> GSHMEILWNEAKAFIAECYQELGKEEEVKDRLDSIKSEIDRTGSYVHTKEELEHGAKMAWRNSNRCIGRLFWNSLNVIDRRDVRTKEDVRDALFHHIETATNNGKIRPSITIFPPEEKGEKQVEIWNHQLIRYAGYESDGERIGDPASRSLTAACEQLGWRGERTDFDLLPLIFRMRGDEQPVWYELPRSLVIEVPITHPDIEAFSDLELKWYGVPIISDMKLEVGGIHYNAAPFNGWYMGTEIGARNLADEKRYDKLKKVASVIGISTNYNTDLWKDQALVELNKAVLYSYKKQGVSIVDHHTAASQFKRFEEQEEEAGRKLTGDWTWLIPPIS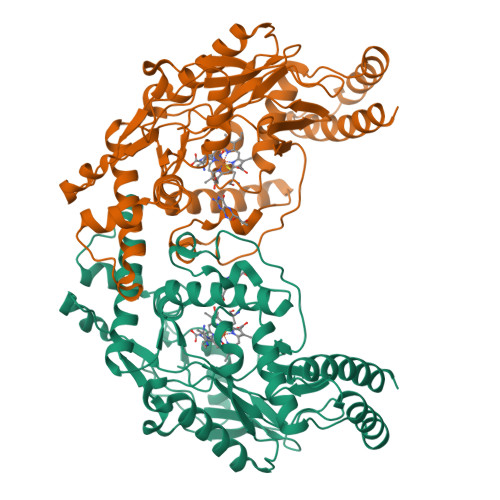PAATHIFHRSYDNSIVKPNYFYQDKPYE All BoNTs are naturally co-expressed with a protective partner protein (NTNH) with which they form a 300 kDa complex, to resist acidic and proteolytic attack from the digestive tract. We have previously identified a new botulinum neurotoxin serotype, BoNT/X, that has unique and therapeutically attractive properties. We present the cryo-EM structure of the BoNT/X-NTNH/X complex and the crystal structure of the isolated NTNH protein. BoNTs are 150 kDa proteins and consist of three domains: the 50 kDa catalytically active light chain (LC) and the 100 kDa heavy chain that is further divided into the translocation domain (HN) and the receptor-binding domain (HC).

In contrast to free BoNT/X, NTNH/X exhibited high thermal stability in the toxin-free state, demonstrated by nanoDSF curves with late unfolding onsets and single, sharp inflection points over a broad pH range with the highest melting temperature of 49.5 °C at pH 6.5. NTNH/X was also stable at high protein concentration (over 40 mg/ml). We determined its structure by X-ray crystallography at the resolution of 3.3 Å. Although the electron density map was not well defined for many side chains, we were able to build the complete main chain, including regions missing in the cryo-EM model. The overall structure of NTNH/X in the free state is very similar to that in the BoNT/X-NTNH/X complex, exhibiting the same domain organization with only a slight difference in the angle between the nLC-nHN portion and the nHC domain. The structures of the individual subdomains of NTNH/X only differ between the free and toxin-bound states locally, in certain loop regions involved either in the toxin-NTNH interface or in crystal contacts. The high stability, relative rigidity, and domain arrangement of NTNH/X support its function as a structural scaffold for BoNT/X. However, NTNH/X has an extended loop with exposed hydrophobic residues, structurally close to the NTNHA nLoop. This loop (NTNH/X residues 128–138) could not be built in the cryo-EM model of the complex, but was built in the X-ray model of free NTNH/X where it extends into the solvent. Although not conserved in other orfX-type NTNH proteins, its position suggests a potential interaction site with other proteins.

> MDINDKLSIDSPIDNKNIIEFITFRTDTSGIQKKIKAYQIAKHIWVVPERYYAEPLNISDEYKIDGGIYNENYLTTDKERQEYLDAICILFKRINNVIEGKKLLSLLSSASPFPFKDDTNKYLLKEALLYVNEENFEFKFFTSNIILFGPGTNISKNQVLPLNGDDATSGVGSVSEICYNPFFTKKFGEYSLDPVIGLIECLLKSLYNLYGIKVSDDIKIPYKLQRALNTDKYSYINLEEALIFGGNDYKIFTEKPYWLSNDYFLKSLNTFEENKAKYEKDLKNDPNLNNELNQYLQQKYSFSISKIWSLNLTAFADIFNINIPTSFLASITFWDRSQYYKINYPNDYNIDGFVNGQWNTNLKNIEKDNNFIIFDKPKQIITYINDIFNLRYTSNLYEDNLDIESNNYYLNFMFEYDKGNNFTINQYKALLDTLDNDFIDSLPPIQGMNAQNKLTSLPIISKGTDTENINSELLLPIHYLKSQTYNLDMYSSIKFTTNIYEVVSEKNSELVYTFLPHINEIMENYSINNTIKTEEEFYNWMENLFINYSIDILEKRNSIIPGITAVLPWIGKALNILNTNNDFEEELQLSGIKGLIKEYENFIIPDMIVPDIPLDNMPRTYDDIDKKLSEIYTKNKFLFLKGYYFIVQEWWTTYYIQFIELKYLCSGAINKQQQLLITVLEKQLFYFTNNGLFPFDAMERMINEFNRSIDIFSRISQQALNNVDIFINECALFIFNNEVYPLFLNNVENNINKANDNVLNYINKATSLTEEQIKELTVKYTFSSIAEVEFFNESYFKKITNMDIKNILTNIKNINNLILSGSQINDDITIFDESGNNLNIKFDPSIRIVDGHTNVAFKLDKSSQYINIPTENINFSFMESFSIDFWLKILDSTESTTLLNCIEDDIGWKLSIQNNNLLWEMKDNLGNNFTSLFTFNINNIWHNITLSIDRLTNTFNCFLDGKLINTDNISNIFSLETNTPIEIQSDNGAILLEAFSILNYPLQQQEVLNRYREAFSNNYTRNYYGDILKYNENYQLYNKTSPDKEVKKVFTNDKDYIAIEYNQNTNNPTFFSLIQKEQSKIYVEENDEVYICVQGDPLNYITIDNNQAVLTKDINLATSFKLKTNLNKPNSLIFSENSQALRLSNRLNDENYILLDLVSKLDDEPLNIFYWEFI>[2x]MNLPTAQEVQGLMARYIELVDVGDIEAIVQMFADDATVEDPFGQPPIHGREQIAAFFR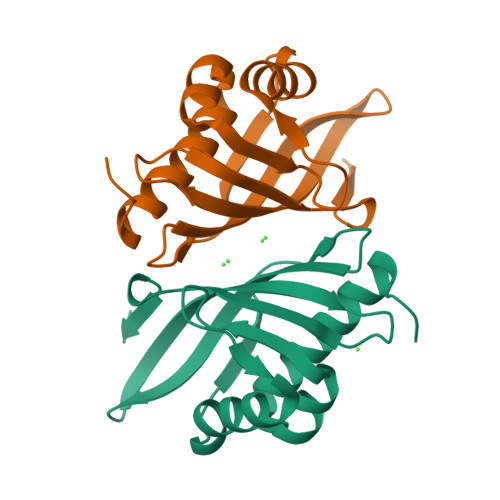QGLGGGKVRACLTGPVRASHNGCGAMPFRVEMVWNGQPCALDVIDVMRFDEHGRIQTMQAYWSEVNLSVREPQ>GARGGSDLEIDNEGVIEADTDAPQEMGDENAEITEAMMDEANEKKGAAIDALNDGELQKAIDLFTDAIKLNPRLAILYAKRASVFVKLQ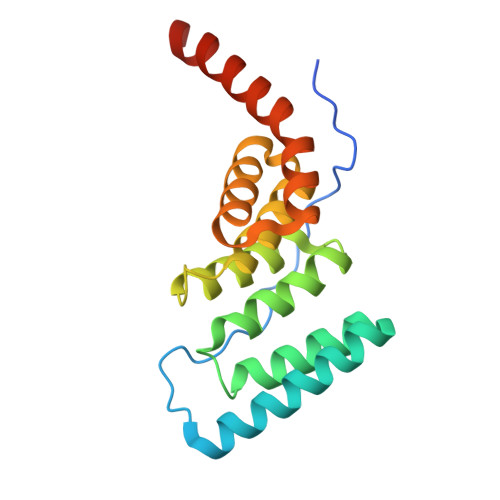KPNAAIRDCDRAIEINPDSAQPYKWRGKAHRLLGHWEEAARDLALACKLDYDEDASAMLREVQPRAQKIAEHRRKYERKREEREIK[4x]> ANKVIQLQKIFQSSTKPLWWRHPRS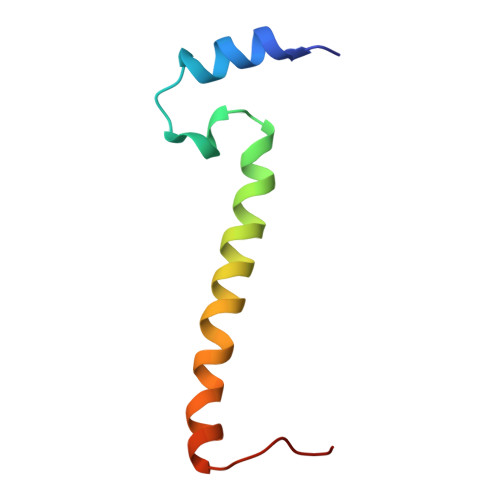ALYLYPFYAIFAVAVVTPLLYIPNAIRGIKAKKA> DSF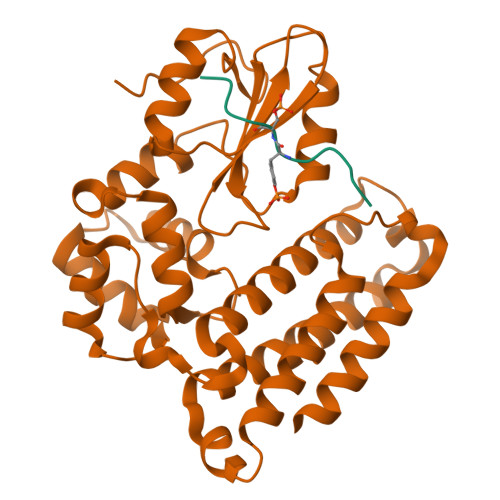LQRYSSDPT;> GSLIGLMKDAFQPHHHHHHHLSPHPPGTVDKKMVEKCWKLMDKVVRLCQNPKLALKNSPPYILDLLPDTYQHLRTILSRYEGKMETLGENEYFRVFMENLMKKTKQTISLFKEGKERMYEENSQPRRNLTKLSLIFSHMLAELKGIFPSGLFQGDTFRITKADAAEFWRKAFGEKTIVPWKSFRQALHEVHPISSGLEAMALKSTIDLTCNDYISVFEFDIFTRLFQPWSSLLRNWNSLAVTHPGYMAFLTYDEVKARLQKFIHKPGSYIFRLSCTRLGQWAIGYVTADGNILQTIPHNKPLFQALIDGFREGFYLFPDGRNQNPDLTG>[3x]MPKYERTYTTQANFILHGGDYNPDQWLDRPDILQADLELMKLSHTNTFTVGVFAWSALEPEEGVYRFEWLDKVFDDIYRIGGRVILATPSGARPAWLSQKYPEVLRVNAARVRQLHGGRHNHCFTSSVYREKTQHINRLLAERYGDHPALLMWHVSNEYGGECHCNLCQEAFREWLKKKYNHDLDALNAAWWTSFWSHTYTDWSQIESPSPIGEHTIHGLNLDWKRFVTDQTISFFENEIVPLRELTPHIPITTNFMADTHDLIPFQGLDYSKFAKHLDVISWDAYPAWHNDWESTADLAMKVGFINDLYRSLKQQPFLLMECTPSLVNWHKVNKAKRPGMHFLSSMQMIAHGSDSILYFQWRKSRGSFEKFHGAVVDHDNRTDSRVFQEVAEVGKALKKMSGIVGTNRPAEV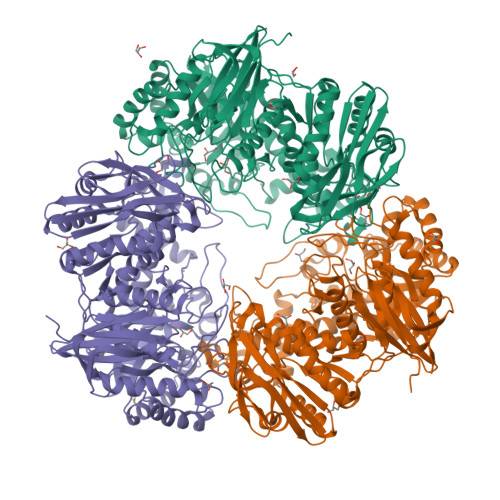AILYDWENNWALNDAQGFAAETKRYPQTLVQHYRPFWERDIPVDVITKEHDFSRYKLLIAPMLYLVSEETIARLKEFVANGGTLVMTYISGIVDEHDLAYLGGWHQDLREMFGMEPIETDTLYPRDRNSVHYRGRSYELKDYATVIKIHAATVEGVYEDDFYADTPAVTSNQYGKGQAYYIGGRLEDQFHRDFYQELMEKLDLRPVLFVKHEKGVSVQARQAPECDYVFIMNFTEEKQAVVLEEKVKDLFTGEEIVGEIMLDKYEVRVVEKRR[(2S,3R)-2-formyl-1-{[4-(methylamino)butyl]carbamoyl}pyrrolidin-3-yl]sulfamic acid | C11 H22 N4 O5 S | 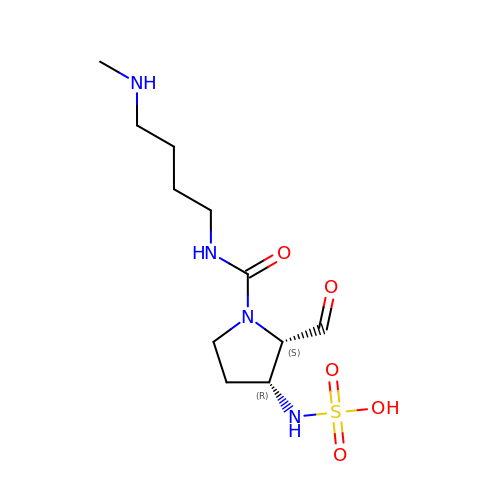KICDPLXBZKSLNF-NXEZZACHSA-N> SMRSIPELRLGVLGDARSGKSSLIHRFLTGSYQV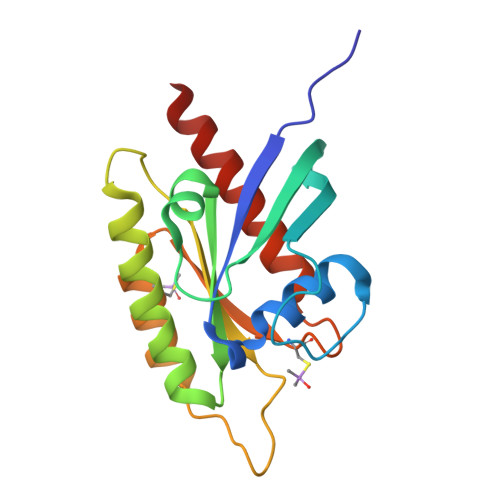LEKTESEQYKKEMLVDGQTHLVLIREEAGAPDAKFSGWADAVIFVFSLEDENSFQAVSRLHGQLSSLRGEGRGGLALALVGTQDRISASSPRVVGDARARALCADMKRCSYYETCATYGLNVDRVFQEVAQKVVTLRKQQQLLA(3S)-4-{[4-(BUT-2-YNYLOXY)PHENYL]SULFONYL}-N-HYDROXY-2,2-DIMETHYLTHIOMORPHOLINE-3-CARBOXAMIDE | C17 H22 N2 O5 S2 | 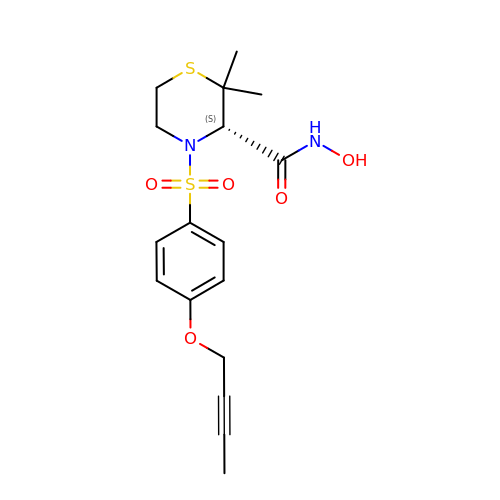CVZIHNYAZLXRRS-HNNXBMFYSA-N>GVALGATRVIYPEGQKQVQLAVTNNDDKSSYLIQSWIENAEGKKDARFVITPPLFSMQGKKENTLRIIDATNGQMPEDRESLFWVNVKAIPAMDKAKTGENYLQFAIVSRIKLLYRPQGLVIPPEQAPGKLEFTRENGGLTLFNPTPYYLT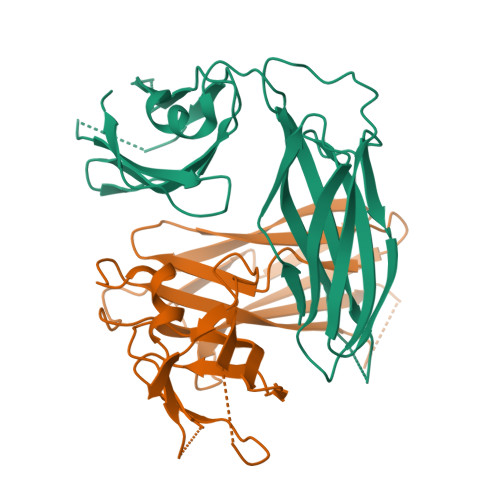VTDLKAGNKSLENTMVPPQGKVTVNIPGGYTGGDITYKTINDYGALTEQVRGVVK[2x]> XADFDAVLKCWGPVEADYTTIGGLVLTRLFKEHPETQKLFPKFAGIAQADIAGNA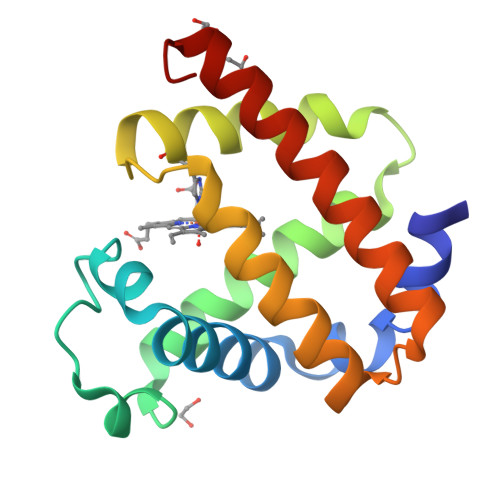AVSAHGATVLKKLGELLKAKGSHAAILKPLANSHATKHKIPINNFKLISEVLVKVMQEKAGLDAGGQTALRNVMGIIIADLEANYKELGFSG> MPSTYKTPGVYIEEISKFPPSIAQVETAIPAFIGYTQIAKVGVENFHTDADNLILRPVRITSLLEYEQFFGKAINETTIQVVIQDTTDSRGN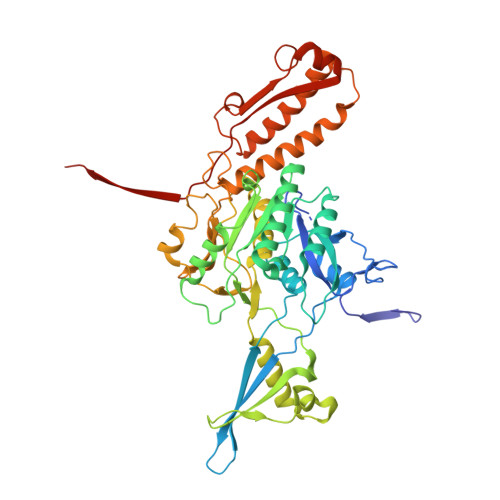LTERKASARITSPSPHNLYYSMQAYFANGGGPCYIVSVGPMSNTGTIQLEALQNGLAEVAKEDEVTLLVFPESQSLSDENYAALMSAALEQCANLQDRFTVMDLKLPATRPIPANAIVGASNAFRDLSLPQDNLKYGACYAPDIETIFNYFYQEDAVTIFRSVNGGAEEQDTLTMAGYNPANGGDGIQYALIESAIDQLPLILPPSPLVVGQYARTDNTRGVWKAPANVALSSVIKPVLKITNEQQNNLNVHPTGKSINAIRAFTGKGTLIWGARTLAGNDNEWRYVSVRRFFNMAEESIKKGSEPFVFEPNDANTWTKVKAMIENFLTLQWRAGALAGAKPEQAFYVKIGLNETMTALDILEGRMIVEIGMAVVRPAEFIILKFSHKMQES>[2x]MVSK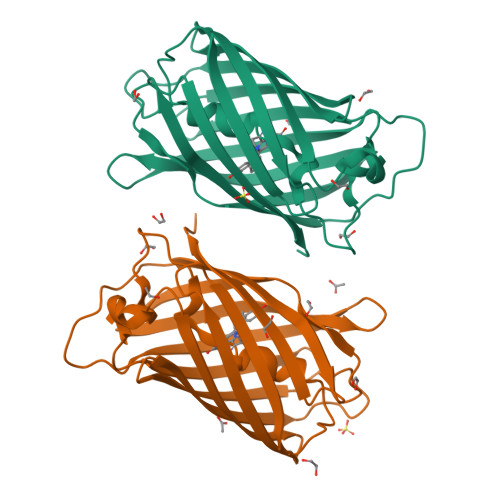GEELIKEEMPMKVVLEGTVNGHQFKCTGEGEGRPYEGVQTMRIKVIEGGPLPFAFDILATSFMYGSRTFVKHPKGIPDYFKQSFPEGFTWERVMRFEDGGVVTVTQDTSLQDGVLIYNAKVRGVNFPSNGPVMQKKTKGWEPNTEMIYPADGGLRGYTDMALKVDGGGHLHCSFVTEYRSKKTVGNIKMPGVYAIDHRLERIEESDNETYVVQREVAVAKYSNLGGGMDELYK> SGKAVDGDTLVLTKEFGLIKIKELYEKLDGKGRKIVEGNEEWTELEKPITVYGYKDGKIVEIKATHVYKGVSSGMVEIRTRTGRKIKVTPIHRLFTGRVTKDGLILKEVMAMHVKPGDRIAVVKKIDGGEYIKLDSSNVGEIKVPEILNEELAEFLGYLMANGTLKSGI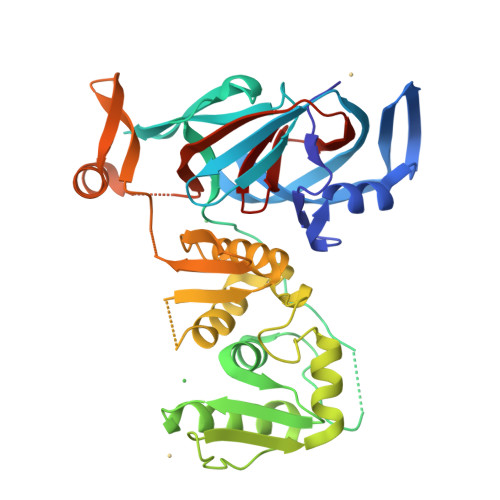IEIYCDDESLLERVNSLSLKLFGVGGRIVQKVDGKALVIQSKPLVDVLRRLGVPEDKKVENWKVPRELLLSPSNVVRAFVNAYIKGKEEVEITLASEEGAYELSYLFAKLGIYVTISKSGEYYKVRVSRRGNLDTIPVEVNGMPKVLPYEDFRKFAKSIGLEEVAENHLQHIIFDEVIDVRYIPEPQEVYDVTTETHNFVGGNMPTLLHN> MPTVVVMDVSLSMTRPVSIEGSEEYQRKHLAAHGLTMLFEHMATNYKLEFTALVVFSSLWELMVPFTRDYNTLQEALSNMDDYDKTCLESALVGVCNIVQQEWGGAIPCQVVLVTDGCLGIGRGSLRHSLATQNQRSESNRFPLPFPFPSKLYIMCMANLEELQSTDSLECLERLIDLNNGEGQIFTIDGPLCLKNVQSMFGKLIDLAYTPFHAVLKCGHLTADVQVFPRPEPFVVDEEIDPIPKVINTDLEIVGFIDIADISSPPVLSRHLVLPIALNKEGDEVGTGITDDNEDENSANQIAGKIPNFCVLLHGSLKVEGMVAIVQLGPEWHGMLYSQADSKKKSNLMMSLFEPGPEPLPWLGKMAQLGP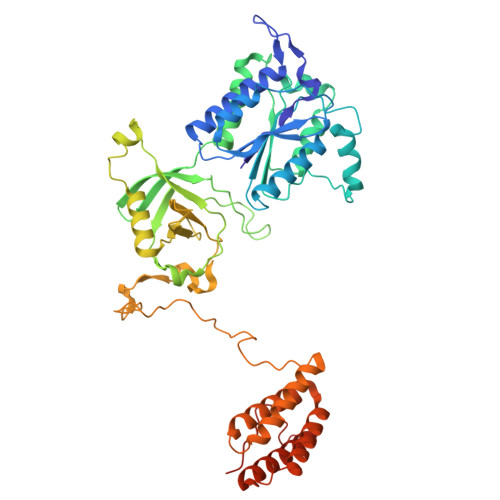ISDAKENPYGEDDNKSPFPLQPKNKRSYAQNVTVWIKPSGLQTDVQKILRNARKLPEKTQTFYKELNRLRKAALAFGFLDLLKGVADMLERECTLLPETAHPDAAFQLTHAAQQLKLASTGTSEYAAYDQNITPLHTDFSGSSTERI>[2x]TGRQEVRAESQFPGTRRPVSATIPGNFAAYHELWRNAFQEIMNDPRHQLHRNDVEYKKIHAIRTVLDDYTKGGNTWWAKFRRIFTFHWNRHHVKVVDDIVKEIDAGNYTTSRALVDRLDNLAISLGSKLNPKGTLKEQIGFIKIQEQNPVEEIENLSRPNLT

Among all bacterial pathogens, Legionella pneumophila maintains the largest known set of translocated substrates, delivering over 300 proteins to the host cell via its Type IVB, Icm/Dot translocation system. In at least nine instances, this regulation is direct—a hallmark of an emerging class of proteins called metaeffectors, or “effectors of effectors”. Through detailed structural and functional analysis, we show that metaeffector activity derives from a diverse range of mechanisms, shapes evolution, and can be used to reveal important aspects of each cognate effector's function. After release into the host cell, translocated bacterial substrates (effectors) regulate one another through several different functional interactions: indirectly, through counteracting modification of a shared host target, or directly through either steric complex formation or direct modification of one effector by another.

To define the mechanism of LegL1 inhibition of RavJ, we first solved the crystal structure of the N‐ and C‐terminal portions of RavJ spanning amino acid residues 1–228 and 251–371, respectively (Table EV4). Structures for amino acid residues 1–228 and 251–371 of RavJ were solved separately to a resolution of 1.3 and 1.9 Å, respectively. The C‐terminal domain of RavJ did not reveal any structural similarity to known proteins or functional domains, but we identified a short conserved motif (H316‐WNRHH‐V322) that is present in another IDTS, WipB, as well as several non‐Legionella proteins. A conserved motif (highlighted in gray) is located in the C‐terminal domain with surface exposed residues H316, R319, and H320. While expression of full‐length RavJ showed a severe growth defect in a spot dilution assay, mutation of each of the putative catalytic residues or the adjacent W172 to alanine fully relieved toxicity as did substitutions in the conserved C‐terminal motif. Septins and elongator complex proteins were identified only with full‐length RavJ and the (230–391) C‐terminal domain, suggesting that the C‐terminal domain is a substrate‐binding domain. Use of the otherwise full‐length loop mutant (H316A/R319A/H320A) as bait abrogated these interactions.>MENFPTEYFLNTTVRLLEYIRYRDSNYTREERIENLHYAYNKAAHHFAQPRQQQLLKVDPKRLQASLQTIVGMVVYSWAKVSKECMADLSIHYTYTLVLDDSKDDPYPTMVNYFDDLQAGREQAHPWWALVNEHFPNVLRHFGPFCSLNLIRSTLDFFEGCWIEQYNFGGFPGSHDYPQFLRRMNGLGHCVGASLWPKEQFNERSLFLEITSAIAQMENWMVWVNDLMSFYKEFDDERDQISLVKNYVVSDEISLHEALEKLTQDTLHSSKQMVAVFSDKDPQVMDTIECFMHGFVTWHLCDRRYRLSEIYEKVKEEKTEDAQKFCKFYEQAANVGAVSPSEWAYPPVAQLANVRSK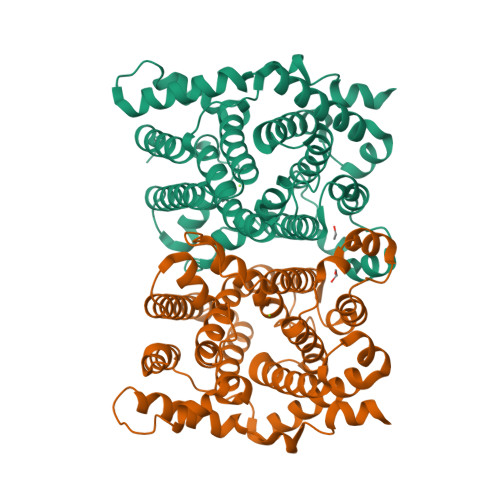DVKEVQKPFLSSIELVE[2x]> DSGQKTVQKILEEVRILEQIGVSHDAQIQELSEMWRVNQQFVTRLQQQLVDIRQTCSRPCQDTTANKISPITGKDCQQVVDNGGKDSGLYYIKPLKAKQPFLVFCEIENGNGWTVIQHRHDGS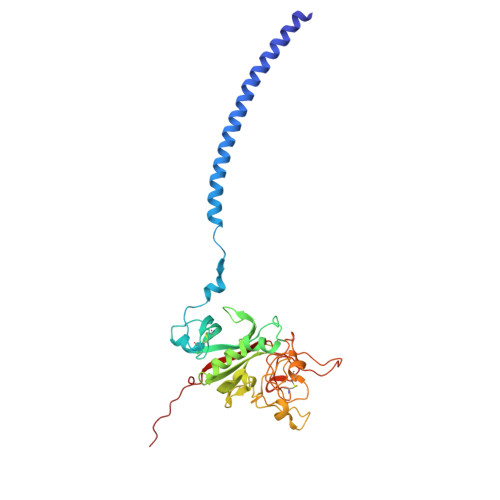VNFTRDWVSYREGFGYLAPTLTTEFWLGNEKIHLLTGQQAYRLRIDLTDWENTHRYADYGHFKLTPESDEYRLFYSMYLDGDAGNAFDGFDFGDDPQDKFYTTHLGMLFSTPERDNDKYEGSCAEQDGSGWWMNRCHAGHLNGKYYFGGNYRKTDVEFPYDDGIIWATWHDRWYSLKMTTMKLLPMGRDLSGHGGQQQSK> SNAMKDFHFDAISAFENYEIEKMRDGHV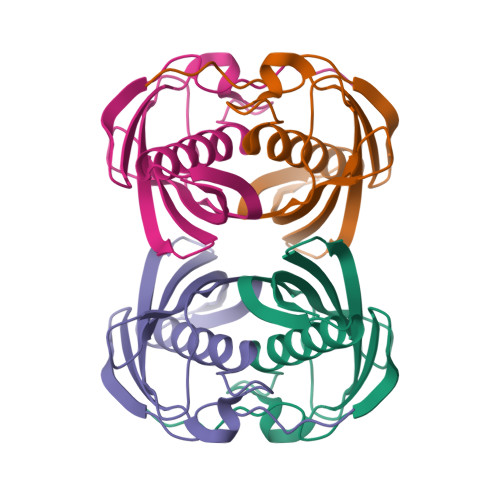VVTTKVVNSSLNYYGNAHGGYLFTLCDQISGLVVISLGLDGVALQSSINYLKAGKLDDVLTIKGECVHQGRTTCVMDVDITNQEGRNVCKATFTMFVTGQRSEERRVRI>[5x]MGSSHHHHHHSQDPLVPRGSWETEERPRTREEECHFYAGGQVYPGEASRVSVADHSLHLSKAKISKPAPYWEGTAVIDGEFKELKLTDYRGKYLVFFFYPLDFTFVCPTEIIAFGDRLEEFRSINTEVVACSVDSQFTHLAWINTPRRQGGLGPIRIPLLSDLTHQISKDYGVYLEDSGHTLRGLFIIDDKGILRQITLNDLPVGRSVDETLRLVQAFQYT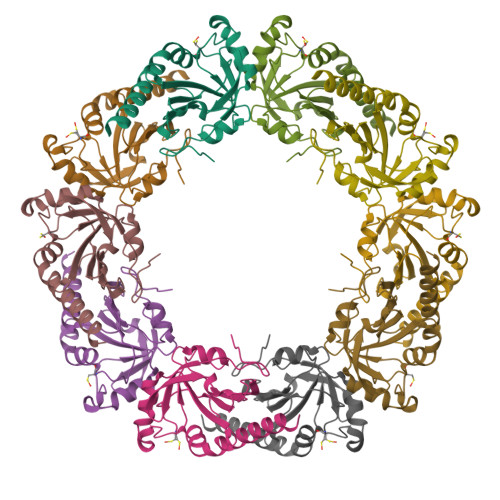DKHGEVAPAGWKPGSETIIPDPAGKLKYFDKLN>SKNRISWVGDAVKTDGKKSYYKKVCIDSETLEVGDCVSVIPDDSSKPLYLARVTALWEDSSNGQMFHAHWFCAGTDTVLGATSD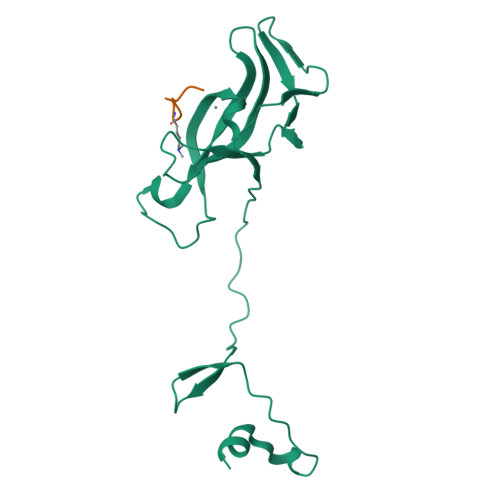PLELFLVDECEDMQLSYIHSKVQVIYKAPSGAGSATYFYQLWYDQDYARFESPPKTQPTEDNKYKFCASCARLA[4x];>[4x]GAKRHRKVLRDNY In this work, we exhaustively probe the ability of all 36 immobile HJ sequences to form DNA crystals in two different designed systems. Three separate self-assembling DNA crystal systems are described in this report: the “4 × 5” and “4 × 6” designs (collectively referred to as the 4 × N systems), and a third construct with a “scrambled” sequence variant of the 4 × 6 lattices. Self-assembly was mediated by three constituent oligonucleotides: (S1) containing four sequence repeats of either 5 or 6 bases; (S2) composed of 21 bases containing complementary regions to both (S1); and (S3) which forms the second junction crossover. The HJ serves as the fundamental component at the core of each unit, and the ultimate assembly of the full lattice is facilitated by the complementary 2-base sticky ends that tail each duplex.

Because the 4 × 6 system yielded R3 symmetry in 5 of 17 junctions, we considered whether the downstream sequences adjacent to the junction could play a role in crystallization efficiency, junction angle, and symmetry preference, or if the HJ alone was the singular determinant. To investigate this possibility, we designed “scrambled” sequences with targeted base substitutions, while maintaining GC content, along each “stem”. Contrary to the buffer preference observed with the native P32 crystals, the scrambled systems exhibited an exclusive preference towards low salt buffers, much like the native R3 crystals. Remarkably, only J1 and J2 retained the P32 symmetry, with all others yielding an R3 lattice. There appeared to be only a marginal difference in the average cell lengths in the R3 scramble crystals (a = b = 113.04 c = 51.10) relative to the native 4 × 6 sequences: the a, b axis trended ~2 Å shorter and c ~1.3 Å longer, whereas in the J1 and J2 cases, the crystals were in good agreement with the original 4 × 6 motif. The average angles of the R3 and P32 crystals were 61.00° (σ = 1.21) and 58.05° (σ = 1.39), respectively. However, in the majority of the crystal structures reported here, the cacodylate anion indeed fits best into the electron density map of our X-ray structures, due to the presence of sodium cacodylate in the crystallization solution. To our knowledge, all experimental structures of HJs in the PDB database reported by diverse independent groups suggest that cations (e.g., Na+, Mg2+, Sr2+, Ba2+) should bind at this location.

> GAACGACAGTGA;> CGCCGACTC;> TCAGCG;> TCGAGTCGCTGTCGT>MPDDAKTANTTTAATTKNAENNRITPVTVIGLGAMGRALAGALLDAGYPTTVWNRTAGRGEDLVARGATLAASPAEAVRAGEVVLVCVVDYAASQAILEPVAADLAGRVLVNVTSDSPERAREAAKWADGHGIRYLDGAVMIPTVMVGSTDALLFYAGDKSAYDEHEQVFTSLGGQSAYVGADHGLAAVYELSMIDFFWTSMSGLVHGYALAAKDGVPATSIAPFLKAHISLLSLLIEVTAKDLDAGEYPGASGNLAAEVEGIEHILHAAELRGLDVSVLRSVRDVARR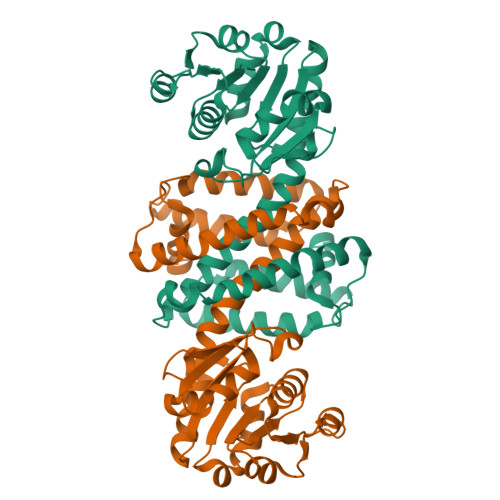AVDLGHGADSWSATVEGARNPA[2x]> MPANDFVSPDSIRAQFSAAMSLMYKQEVPLYGTLLELVSEINQQVMAQQPEVAEALRWTGEIERLDQERHGAIRVGTAEELATIARLFAVMGMQPVGYYDLSSAGVPVHSTAFRAVHEQSLHVSPFRVFTSLLRLELIDNPQLRELAQSILAKRQIFTSRALELIAQCEREGGLDAADAETFVQEALHTFRWHQDATVTAEQYQQLHDQHRLIADVVAFKGPHINHLTPRTLDIDAIQLGMPAKGIPPKAVVEGPPTRRHPILLRQTSFKALQETVAFRDQQGREGSHTARFGEIEQRGAALTPKGRQLYDKLLDATRVALGGAPAEANAERYMALLQANFAEFPDDLAQMREQGLAYFRYFATEKGLAARDQEGRPTTLQGLIDAGHVHFEALVYEDFLPVSAAGIFQSNLGDDAQAEYGSNANREAFEAALGLQVQDELALYAQSERRSLQACAQALNLGSM

In this step, 2OA is converted to D-2-hydroxyglutarate (2HG) in a reaction catalyzed by the Fe(II)-dependent DUF1338 family enzyme hydroxyglutarate synthase (HglS). Homologs of this enzyme are broadly distributed across multiple domains of life, including nearly every sequenced plant genome. Conversion of 2OA directly to D-2HG requires two discrete chemical steps, a decarboxylation and hydroxylation, making the chemical mechanism of the enzyme puzzling. We further show that despite very low sequence identity, plant homologs also catalyze the conversion of 2OA to 2HG and adopt the same structural fold as the bacterial enzyme, suggesting that DUF1338 family proteins catalyze the last unknown step of plant lysine catabolism.

To better understand the unusual HglS reaction, we obtained crystal structures of the enzyme both with and without a bound substrate. Initially, Hg1S was crystallized without substrate, and the Hg1S structure was solved at 1.1 Å resolution. Further analysis also revealed the presence of a metal cofactor bound within a conserved metal cofactor-binding motif—consisting of the residues His 70, His 226, and Glu 294—common to the DUF1338 structures. HglS and HMS structure comparison revealed the two enzymes share a similar central β-sheet fold common to the DUF1338 structures. To determine metal cofactor identity within the HglS structure, we conducted a fluorescent scan of a HglS crystal. We detected a photon emission near 7475 eV, the K-alpha emission of nickel. In addition, a less intense peak corresponding to the K-alpha emission of iron was also observed. We therefore assigned the co-crystallized metal as Ni(II) with a small percent Fe(II) occupancy. While the metal cofactors present in the HMS and HglS structures differ, we previously determined that HglS utilizes Fe(II), not Ni(II), for catalysis. The nickel bound to HglS is likely derived from the nickel affinity chromatography protein purification.> GTHLLFAQTGKIERLPLERNTMKKTEAKAFLHIPAKVIIGLAFDCVDKVVYWTDISEPSIGRASLHGGEPTTIIRQDLGSPEGIALDHLGRT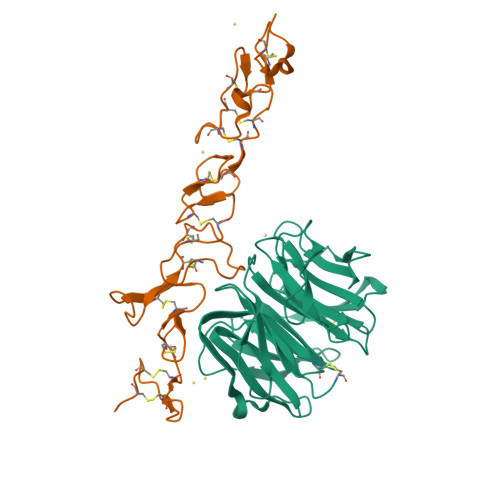IFWTDSQLDRIEVAKMDGTQRRVLFDTGLVNPRGIVTDPVRGNLYWTDWNRDNPKIETSHMDGTNRRILAQDNLGLPNGLTFDAFSSQLCWVDAGTHRAECLNPAQPGRRKVLEGLQYPFAVTSYGKNLYYTDWKTNSVIAMDLAISKEMDTFHPHKQTRLYGITIALSQCPQGH;> QPCPCPGGSSCAIVPKTKEVVCTHCPTGTAGKRCELCDDGYFGDPLGSNGPVRLCRPCQCNDNIDPNAVGNCNRLTGECLKCIYNTAGFYCDRCKEGFFGNPLAPNPADKCKACACNPYGTVQQQSSCNPVTGQCQCLPHVSGRDCGTCDPGYYNLQSGQGCER> MNNDNPLFKSAMVALSLKISIGNVVKTMQFEPSTMVYDACRMIRERIPEALAGPPNDFGLFLSDDDPKKGIWLEAGKALDYYMLRNGDTMEYRKKQRPLKIRMLDGTVKTIMVDDSKTVTDMLMTICARIGITNHDEYSLVRELMEEKKDELNW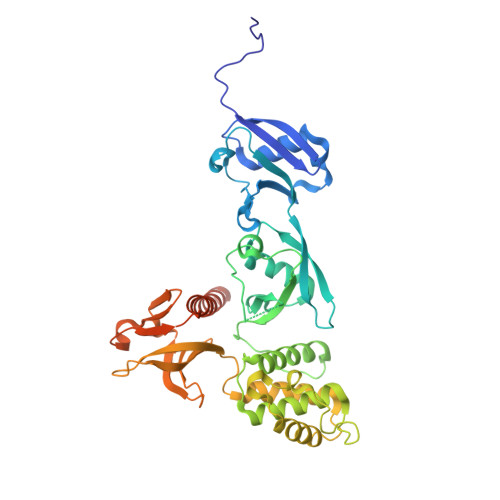LDHGRTLREQGVEEHETLLLRRKFFYSDQNVDSRDPVQLNLLYVQARDDILNGSHPVSFDKACEFAGFQCQIQFGPHNEQKHKAGFLDLKDFLPKAAVKQKGERKIFQAHKNCGQMSEIEAKVRYVKLARSLQTYGVSFFLVKEKMKGKNKLVPRLLGITKECVMRVDEKTKEVIQEWSLTNIKRWAASPKSFTLDFGDYQDGYYSVQTTEGEQIAQLIAGYIDIILKKKKSKDHFGLEGDEESTMLEDSVSPKKST1-ETHOXY-2-(2-METHOXYETHOXY)ETHANE | C7 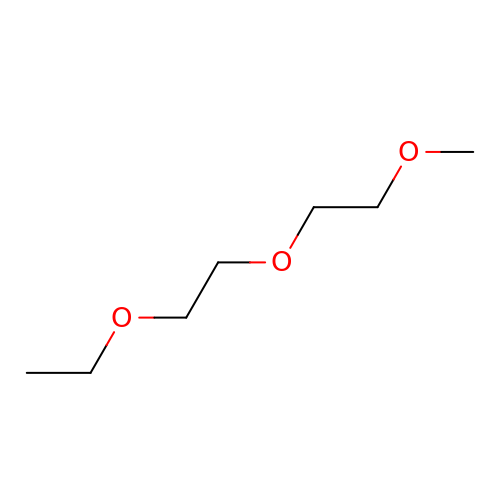H16 O3 | CNJRPYFBORAQAU-UHFFFAOYSA-N> MKLTPKELDKLMLHYAGELARKRKEKGIKLNYVEAVALISAHIMEEARAGKKTAAELMQEGRTLLKPDDVMDGVASMIHEVGIEAMFPDGTKLVTVHTPIEANGKLVPGELFLKNEDITINEGKKAVSVKVKNVGDRPVQIGSHFHFFEVNR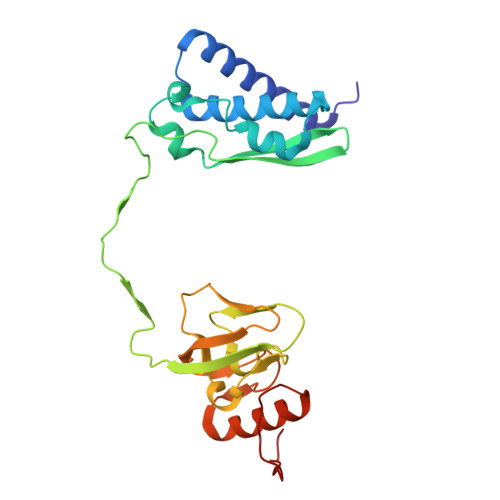CLDFDREKTFGKRLDIASGTAVRFEPGEEKSVELIDIGGNRRIFGFNALVDRQADNESKKIALHRAKERGFHGTKSDDNYVKTIKE>MGSDSIDTPNYDVQKHINKLCGMLLITEDANHKFTGLIGMLYAMSRLGREDTIKILRDAGYHVKANGVDVTTHRQDINGKEMKFEVLTLASLTTEIQINIEIESRKSYKKMLKEMGEVAPEYRHDSPDCGMIILCIAALVITKLAAGDRSGLTAVIRRANNVLKNEMKRYKGLLPKDIANSFYEVFEKHPHFIDVFVHFGIAQSSTRGGSRVEGIFAGLFMN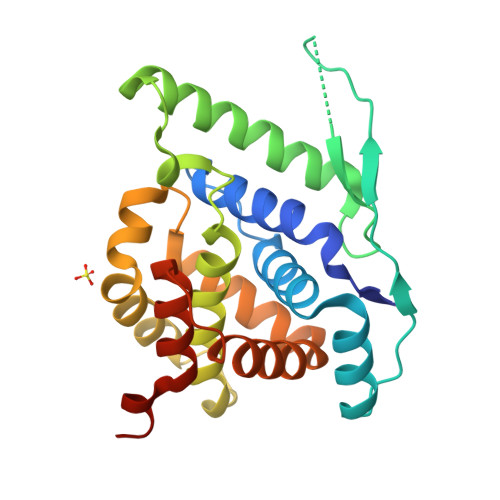AYGLEHHHHHH[2x];>[2x]DLSLEDF>[2x]GSHMAKTYDYLFKLLLIGDSGVGKTCVLFRFSEDAFNSTFISTIGIDFKIRT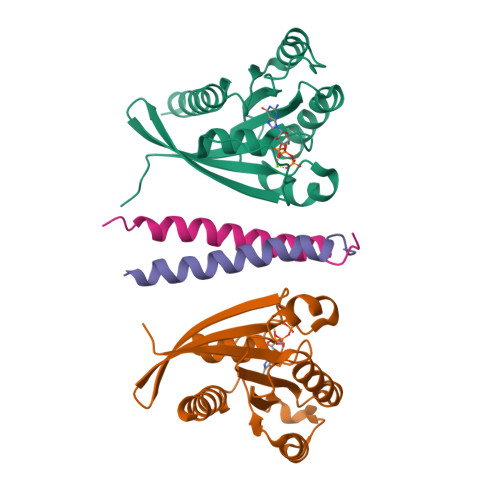IELDGKRIKLQIWDTAGLERFREITTAYYRGAMGIMLVYDITNEKSFDNIRNWIRNIEEHASADVEKMILGNKCDVNDKRQVSKERGEKLALDYGIKFMETSAKANINVENAFFTLARDIKAKMDKKLEGNS;>HHHHHHNRPRFTLQELRDVLQERNKLKSQLLVVQEELQCYKSG[2x]>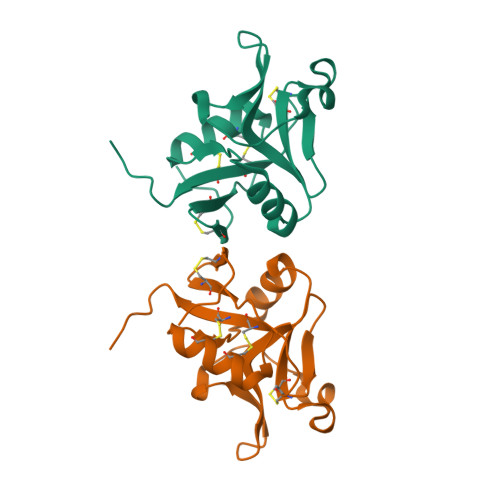[2x]MASGRGFEKYWFCYGIKCYYFVMDRKTWSGCKQTCQISSLSLLKIDNEDELKFLKLLVPSDSYWIGLSYDNKKKDWAWINNGPSKLALNTMKYNIRDGGCMLLSKTRLDNDNCDKSFICICGKRLDKFPH> MARSMSNRSTAKRFISALNNVAERTYNNIFQFHQLRQIAKELNIQVADFENFIGSLNDQGYLLKKGPKVY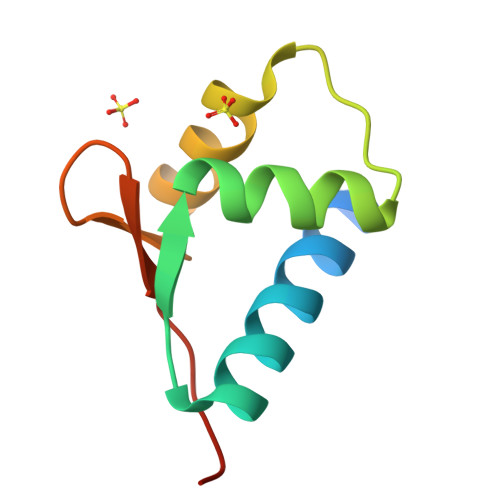QLQTMHHHHHH>MRLWKAVVVTLAFVSTDVGVTTAIYAFSHLDRSLLEDIRHFNIFDSVLDLWAACLYRSCLLLGATIGVAKNSALGPRRLRASWLVITLVCLFVGIYAMAKLLLFSEVRRPIRDPWFWALFVWTYISLAASFLLWGLLATVRPDAEALEPGNEGFHGEGGAPAEQASGATLQKLLSYTKPDVAFLVAASFFLIVAALGETFLPYYTGRAIDSIVIQKSMDQFTTAVVVVCLLAIGSSLAAGIRGGIFTLVFARLNIRLRNCLFRSLVSQETSFFDENRTGDLISRLTSDTTMVSDLVSQNINIFLRNTVKVTGVVVFMFSLSWQLSLVTFMGFPIIMMVSNIYGKYYKRLSKEVQSALARASTTAEETISAMKTVRSFANEEEEAEVFLRKLQQVYKLNRKEAAAYMSYVWGSGLTLLVVQVSILYYGGHLVISGQMSSGNLIAFIIYEFVLGDCMESVGSVYSGLMQGVGAAEKVFEFIDRQPTMVHDGSLAPDHLEGRVDFENVTFTYRTRPHTQVLQNVSFSLSPGKVTALVGPSGSGKSSCVNILENFYPLQGGRVLLDGKPIGAYDHKYLHRVISLVSQEPVLFARSITDNISYGLPTVPFEMVVEAAQKANAHGFIMELQDGYSTETGEKGAQLSGGQKQRVA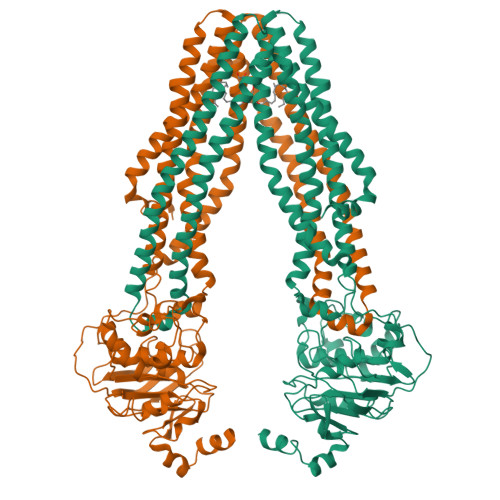MARALVRNPPVLILDEATSALDAESEYLIQQAIHGNLQRHTVLIIAHRLSTVERAHLIVVLDKGRVVQQGTHQQLLAQGGLYAKLVQRQMLGLEHPLDYTASHKEPPSNTEHKA[2x]>MAFADDHAMSPDMKLLAGASNWVNQSGSVAQFVFTPSPTQPQTYEVSGNYINNAQGTGCKGTCYPLSGAYYSGNQIISFSVVWSNASANCQSATGWTGYFDFSGSQAVLKTDWNLAFYSGSTPAIQQGQDDFMQS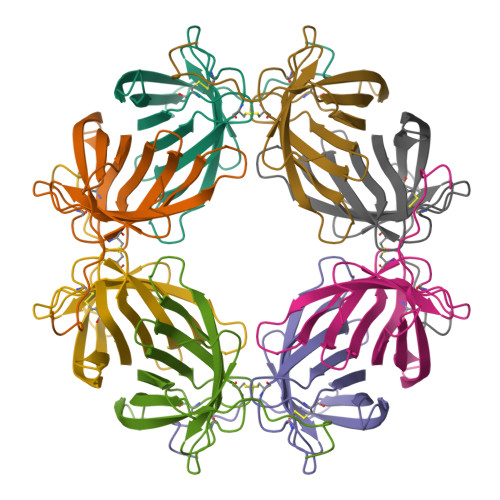VATVSESLLTE[2x]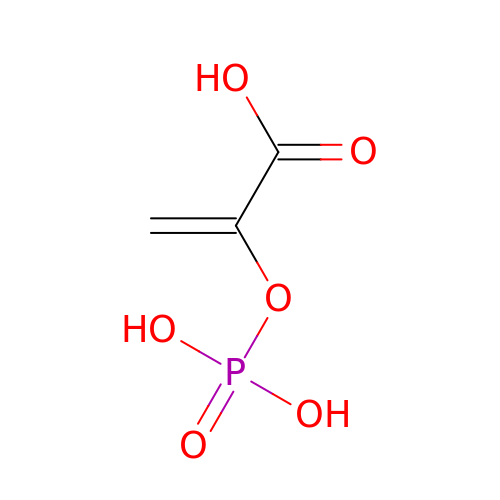PHOSPHOENOLPYRUVATE | C3 H5 O6 P | DTBNBXWJWCWCIK-UHFFFAOYSA-N MK catalyzes the fourth step in the MVA pathway, the transfer of the ATP γ-phosphoryl onto (R)-MVA to give (R)-MVA 5-phosphate. The enzyme is, along with galactokinase (GK), homoserine kinase (HSK), MK and PMK, a founding member of the GHMP kinase superfamily. LmMK exhibits the characteristic GHMP kinase fold consisting of two domains. High-resolution crystal structures of LmMK are reported and provide, for the first time, insight into the binding of substrate by any MK.

Recombinant LmMK and a selenomethionine (SeMet) derivative produced ordered, isomorphous monoclinic crystals and a single-wavelength anomalous dispersion (SAD) experiment provided initial phase information to solve the structure. The SAD approach was required because molecular replacement calculations using known MK structures failed. Although the non-hydrolysable ATP analogue adenosine 5'-(β,γ-imido) triphosphate (AMPPNP) and (R/S)-MVA were included in crystallization solutions there was no indication of ordered ligand binding. There are two molecules in the asymmetric unit (A and B) related by a non-crystallographic (NCS) two-fold axis of symmetry and the surface area between the two is 930 Å2 per molecule, only 6% of the total surface area of the protein. Such a low value is consistent with results from gel filtration and ultracentrifugation experiments that indicate LmMK is a monomer in solution. Molecules A and B overlay with an r.m.s.d. of 1.2 Å for all atoms. Molecule A of LmMK binds the substrate and overlays on the apo-enzyme molecule A with an r.m.s.d. of 0.7 Å for all atoms. This indicates that there no large-scale conformational changes result from substrate binding and the molecules are so similar that it is only necessary to detail molecule A. The replacement of the insert and two helical segments in the rat enzyme with the short loop connecting β3-α2 in LmMK results in a polypeptide conformation, not observed in structures of GHMP kinases, that lies across and restricts access to the ATP binding cavity. Despite our efforts, extending to the complete structural analysis of several diffraction datasets (not shown), we were unable to obtain a binary structure of LmMK in complex with ATP, any nucleotide, or a ternary dead-end complex.

>[2x]GSHMSKPVKSKTTGKNIGYGKVILFGEHFVVHGAEAIVAGISEYTECRLEINPGVPGLQVDDQRPAIPGYIAQKRDEQIKAHQLVLDHLKVDLSGDGLKMFIGGPLVPSSGIGASASDVVAFSRALSELYQLNLTDEEVNLSAFVGEGGYHGTPSGADNTAATYGGLILYRRQNGKSVFKPIAFQQRLYLVVVGTGINASTAKVVNDVHKMKQQQPVQFKRLYDNYTHIVSQAREALQKGDLQRLGQLMNANHDLCRQIDVSCRELESIVQTCRTYGALGAKLSGTGRGGIAVALAASSDQRDAIVKGLKAKCPEAKFIWRYTVQPSAASNL>MAMDVTRSQAQTALTLVEQILAEFQLQEEDLKKVMRRMQKEMDRGLRLETHEEASVKMLPTYVRSTPEGSEVGDFLSLDLGGTNFRVMLVKVGEGEEGQWSVKTKHQMYSIPEDAMTGTAEMLFDYISECISDFLDKHQMKHKKLPLGFTFSFPVRHEDIDKGILLNWTKGFKASGAEGNNVVGLLRDAIKRRGDFEMDVVAMVNDTVATMISCYYEDHQCEVGMIVGTGCNACYMEEMQNVELVEGDEGRMCVNTEWGAFGDSGELDEFLLEYDRLVDESSANPGQQLYEKLIGGKYMGELVRLVLLRLVDENLLFHGEASEQLRTRGAFETRFVSQVESDTGDRKQIYNILSTLGLRPSTTDCDIVRRACESVSTRAAHMCSA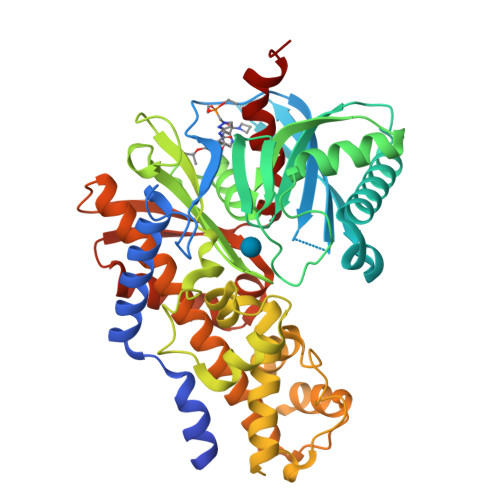GLAGVINRMRESRSEDVMRITVGVDGSVYKLHPSFKERFHASVRRLTPSCEITFIESEEGSGRGAALVSAVACKKACMLGQ[2x]>DIFNRDPRDHYDLLQRLGGGTYGEVFKARDKVSGDLVALKMVKMEPDDDVSTLQKEILILKTCRHANIVAYHGSYLWLQKLWICMEFCGAGSLQDIYQVTGSLSELQISYVCREVLQGLAYLHSQKKIHRDIKGANILINDAGEVRLADFGISAQIGATLARRLSFIGTPYWMAPEVAAVALKGGYNEL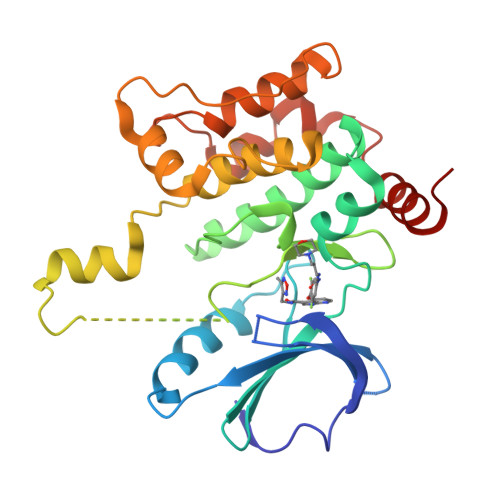CDIWSLGITAIELAELQPPLFDVHPLRVLFLMTKSGYQPPRLKEKGKWSAAFHNFIKVTLTKSPKKRPSATKMLSHQLVSQPGLNRGLILDLLDKLKNPG[2x]>[8x]MASSHHHHHHSSGLVPRGSSMGHNKKFDRSEHVYRNDSFLELIKDAVR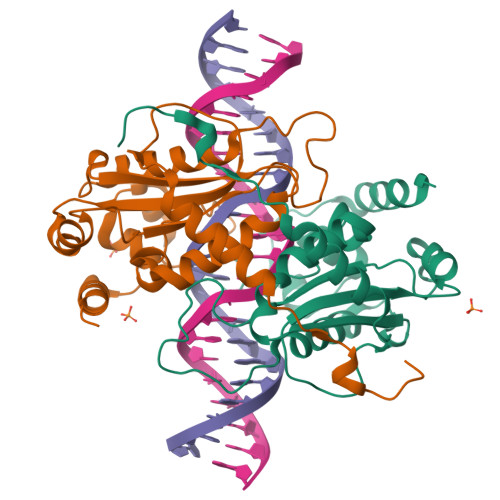FFSGTPVHSLPPPERFQGAGVFALYYTGHYSLYDEYSRINRKAYNLPIYVGKAVPAGWRQSRISDHETRAGSELSNRIREHGRNIAKTSNLDLCDFSCRFVIFEATGSDMISTVEAALIKIYKPLWNTVVDGFGNHTPGAGRFAQAKSDWDVIHPGREWAEKCTGVHSEPYFIEERIKQYFSKSNFT> GGSAPIPDLKVFEREGVQLNLSFIRPPENPALLLITITATNFSEGDVTHFICQAAVPKSLQLQLQAPSGNTVPARGGLPITQLFRILNPNKAPLRL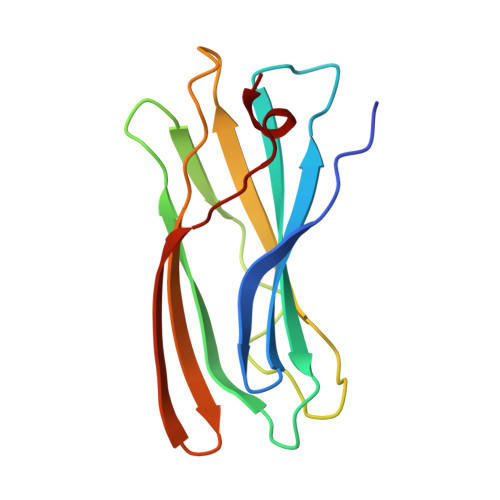KLRLTYDHFHQSVQEIFEVNNLPVESWQ> SMTQFEGFTNLYQVSKTLRFELIPQGKTLKHIQEQGFIEEDKARNDHYKELKPIIDRIYKTYADQCLQLVQLD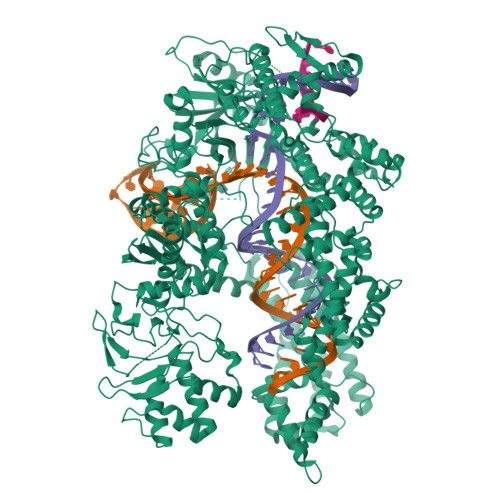WENLSAAIDSYRKEKTEETRNALIEEQATYRNAIHDYFIGRTDNLTDAINKRHAEIYKGLFKAELFNGKVLKQLGTVTTTEHENALLRSFDKFTTYFSGFYENRKNVFSAEDISTAIPHRIVQDNFPKFKENCHIFTRLITAVPSLREHFENVKKAIGIFVSTSIEEVFSFPFYNQLLTQTQIDLYNQLLGGISREAGTEKIKGLNEVLNLAIQKNDETAHIIASLPHRFIPLFKQILSDRNTLSFILEEFKSDEEVIQSFCKYKTLLRNENVLETAEALFNELNSIDLTHIFISHKKLETISSALCDHWDTLRNALYERRISELTGKITKSAKEKVQRSLKHEDINLQEIISAAGKELSEAFKQKTSEILSHAHAALDQPLPTTLKKQEEKEILKSQLDSLLGLYHLLDWFAVDESNEVDPEFSARLTGIKLEMEPSLSFYNKARNYATKKPYSVEKFKLNFQMPTLASGWDVNKEKNNGAILFVKNGLYYLGIMPKQKGRYKALSFEPTEKTSEGFDKMYYDYFPDAAKMIPKCSTQLKAVTAHFQTHTTPILLSNNFIEPLEITKEIYDLNNPEKEPKKFQTAYAKKTGDQKGYREALCKWIDFTRDFLSKYTKTTSIDLSSLRPSSQYKDLGEYYAELNPLLYHISFQRIAEKEIMDAVETGKLYLFQIYNKDFAKGHHGKPNLHTLYWTGLFSPENLAKTSIKLNGQAELFYRPKSRMKRMAHRLGEKMLNKKLKDQKTPIPDTLYQELYDYVNHRLSHDLSDEARALLPNVITKEVSHEIIKDRRFTSDKFFFHVPITLNYQAANSPSKFNQRVNAYLKEHPETPIIGIDRGERNLIYITVIDSTGKILEQRSLNTIQQFDYQKKLDNREKERVAARQAWSVVGTIKDLKQGYLSQVIHEIVDLMIHYQAVVVLANLNFGFKSKRTGIAEKAVYQQFEKMLIDKLNCLVLKDYPAEKVGGVLNPYQLTDQFTSFAKMGTQSGFLFYVPAPYTSKIDPLTGFVDPFVWKTIKNHESRKHFLEGFDFLHYDVKTGDFILHFKMNRNLSFQRGLPGFMPAWDIVFEKNETQFDAKGTPFIAGKRIVPVIENHRFTGRYRDLYPANELIALLEEKGIVFRDGSNILPKLLENDDSHAIDTMVALIRSVLQMRNSNAATGEDYINSPVRDLNGVCFDSRFQNPEWPMDADANGAYHIALKGQLLLNHLKESKDLKLQNGISNQDWLAYIQELRN> GSHMEKLAKNKVISIDAGRKYFTLNQLKRIVDKASELGYSDVHLL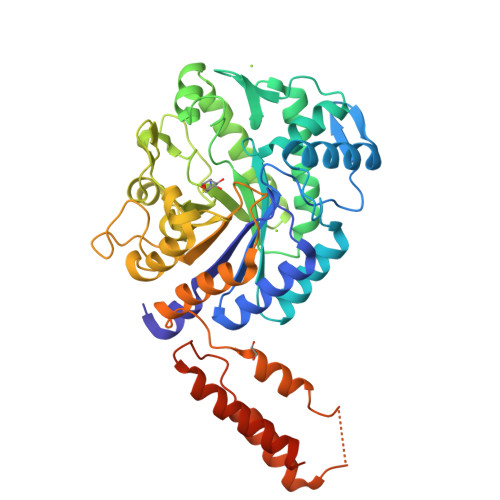LGNDGLRFLLDDMTITANGKTYASDDVKKAIIEGTKAYYDDPNGTALTQAEVTELIEYAKSKDIGLIPAINSPGHMDAMLVAMEKLGIKNPQAHFDKVSKTTMDLKNEEAMNFVKALIGKYMDFFAGKTKIFNFGTDEYANDATSAQGWYYLKWYQLYGKFAEYANTLAAMAKERGLQPMAFNDGFYYEDKDDVQFDKDVLISYWSKGWWGYNLASPQYLASKGYKFLNTNGDWYYILGQKPEDGGGFLKKAIENTGKTPFNQLASTKYPEVDLPTVGSMLSIWADRPSAEYKEEEIFELMTAFADHNKDYFRANYNALREELAKIPTNLEGYSKESLEALDAAKTALNYNLNRNKQAELDTLVANLKAALQGKKPAVTHSGSLDENEVAANVETRP;>[3x]GSHMEKLAKNKVISIDAGRKYFTLNQLKRIVDKASELGYSDVHLLLGNDGLRFLLDDMTITANGKTYASDDVKKAIIEGTKAYYDDPNGTALTQAEVTELIEYAKSKDIGLIPAINSPGHMDAMLVAMEKLGIKNPQAHFDKVSKTTMDLKNEEAMNFVKALIGKYMDFFAGKTKIFNFGTDEYANDATSAQGWYYLKWYQLYGKFAEYANTLAAMAKERGLQPMAFNDGFYYEDKDDVQFDKDVLISYWSKGWWGYNLASPQYLASKGYKFLNTNGDWYYILGQKPEDGGGFLKKAIENTGKTPFNQLASTKYPEVDLPTVGSMLSIWADRPSAEYKEEEIFELMTAFADHNKDYFRANYNALREELAKIPTNLEGYSKESLEALDAAKTALNYNLNRNKQAELDTLVANLKAALQGLKPAVTHSGSLDENEVAANVETRP> EQECT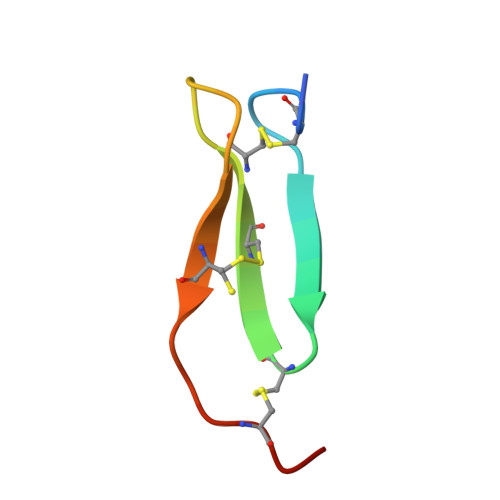PGQTKKQDCNTCNCTPTGVWACTRKGCPPH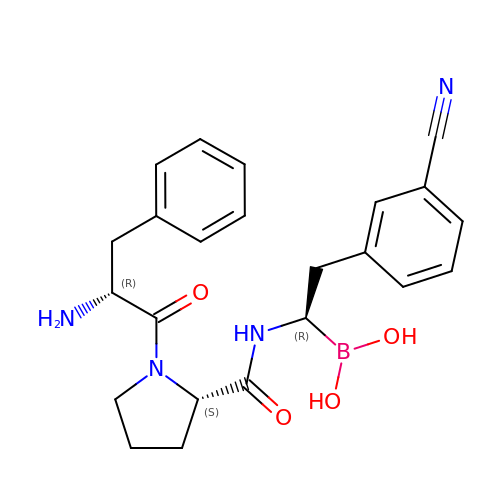1-{[1-(2-AMINO-3-PHENYL-PROPIONYL)-PYRROLIDINE-2-CARBONYL]-AMINO}-2-(3-CYANO-PHENYL)-ETHANEBORONIC ACID | C23 H27 B N4 O4 | UFOIPTZMXQILSG-HKBOAZHASA-N> MLTMKDIIRDGHPTLRQKAAELELPLTKEEKETL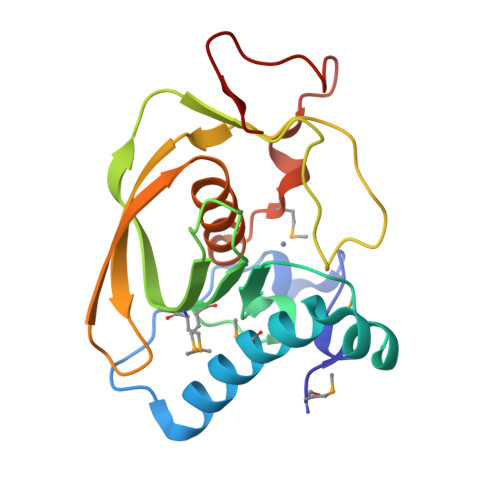IAMREFLVNSQDEEIAKRYGLRSGVGLAAPQINISKRMIAVLIPDDGSGKSYDYMLVNPKIVSHSVQEAYLPTGEGCLSVDDNVAGLVHRHNKITIKAKDIEGNDIQLRLKGYPAIVFQHEIDHLNGVMFYDHIDKDHPLQPHTDAVEVH>[2x]MNILKHFPSYVGPSKIRTLVIPIGHWTRKEFNNAVQKLSEFNEIHLSDVTPIDSPIFTPQGFPHGKLFFDFLTIDHDDALELFLYDFEPFRKTFVIIGLVNDYSDPLTNLNFMKEKYPTLISPNLVYASSTPTKELEQTIDTMENVFASSPDMQKNIETIMCDIARNFLTALNSYYSSYKHVTLRSPGAIGGNAVLKTTLIRQNSYTSSSSSTPMSAVQSSVSSSSKAGSVTTASKRLSSFEMTTNSLKRSASLKLATTLSTSENRSQQKSLGRQMKILGNFQLLAGRYVDALNSFVDAITTLYKVRDYLWLGSALDGISICFLLLSYLGLSYQIPQIVSLICPVEKLNFESSSTGISPVDSNSKATASTTASSTPRNSISIAAMQSPRNSIMSLSAPALNIDVENINLPLLIKCISDKVLYYYDLSLMHNSEYAPQVVYCEFLLKTLTFMTSCYKSSEFSKDVLDNIVKNQHRALSDIPNSPMFPRFEVYFYSNKLFELQLKEMQVEAQIKIYSTMAEVYRLLGYKRKQLFVLRLLMVALLATPNKIAWHPDYRTLIDTIIELLNINESEAKINVDDPSQSTWLILQKKILQLCIKVSRKINDFEYVAKFSSILITKYTHLLNQSEQDALFKEYIQPSITNESITSYWDPFILREVVINRILDSDPTSNEIPLESDVSSLESLENRQKTQDINPQEVFNPFKRVQPTSFVSNNSTKVPILVFLVGDKAEFTCRVQNPFKFDFTINDIQLDEEISEFCEIDRKAVSYSGPYNVKAESIRSITLPLIIKKPTYKKIYEISCLKISILKLPLQKFDIINDSRRSNPVEEEAEYSKCIYGKLKIKILPEQPQLELLSTSKMTRNSWMMLDGTKTDFHITVRNKSLSCAINHIKIIPMNNIEQMLKPDYWKKMPPDDLYIMEKQLDWLSKSCVRIIKLPTVIKPNETITFDLELDNTAVPFNFTGFDLLIEYGMSATDESCIYLKKLSIPYEVTLRRTIEVPSMDIIPLNELFSSQVENVDWIEYVMSKIRAESNLHSRDFILLLLDFRNSWIDGIKLNVQFEDFTSNEYHVEASHTSRIIVPIKKIDYKKYNFENTPIPRIYPGRQFIQSGLNEEQTIEMRQKFWCREHIISKLKCNWKLTTDQSVTGSVDFNKFIEKFDHKMVYTIYPGRLFYGVQLLLDEPKVKVGEIINLKIITEPTSTCRRKQNSTVNFLDIVIFDSKTSKILPRSNRRILYNGSLTKPISTTKVSEINLEIIPIEKGRYEFSVCISKSNNQDGIIQFDSENVILSVI;>MDKEIYCGSVPVSYFDPFDLFESLRPEFQQILPLDNIHWKAFDGTVRTVNRLPIELIPEGRGEADKSNDEQPFIRFLIVNCISIDQYRAKVRPLVRQWLPNLESVSSSTGEKMIYKPIILLYANSEVVDSNLFKSVSLMEKFGKDFPHVQTLEVRSVYRSPKERQEFWNQFSQKIKASVLSIFQKRLTHLQHSLANLQKGNNFEEQLLTREKLYELYVVFNILEDASLELQKIKKEILRRNMNMPDGKLQVPFESSSKSDESLGSIIIEGTLDKFQLHKYFFIRRLRLLKLEDQTLTAFVGAFQLIKNFIESISIEYRKSVRLLEFKHYFITSMLSYFEFENVSNPLLCEIKAELLMLKRDNWVQGVMATSGYRLMDKNYPNSDVKYKFDLLKETFVDETVFQENFLTLTKEILSLFNKCEGKRQRIVDILSIEIGLLYYQGKKYEEAVSLFLSCYEYYTQTNWNSIGLKILQVFIDSLSHCPKLDVLQIDGESVSASAVLTNAFLNILKLCKDNDSKEIWWKKFMDLQMKNNIHLMYPLDGLFEVTLNSKVHLARANVSAIEVNLKSYGFPEDISTKTMRLSLKNMGGDVIVFGASDFLLKKGENKLILECRDIMYGEFSLLSFEIIVEGITFVKEFPENQDEFIVVPEIYCKESTKVLVKQAHNLNLGEYALELKSVQSDALESLQVEVEVQKNIGNMKNLPVSFSMDEIQARKRYNTPFENVRLEYYLLDQITAFDLIIKTSFTKKNDQGTFGETKKVRIQCYLQLSVSVEDIFKKDIFFFKFLLNSSVREEPVILYSSELSAPDTRNDYNIRGDYIATTPALITFDGNESFINCYEITANNNFDSKDIFNLKVRYNTLKEQLDCFITDAVLIEGDVEWFILFEKWKTFWELEILKKLKYDYDAFKENRIIRLLKTS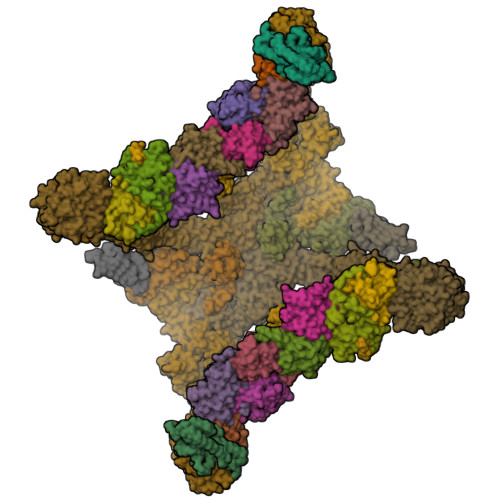IDLNKTKSKIRNLCIEKAVLDKILICLNKVSRGIAVCNTDMDEYVRNLVPKQLTVPVQLPGFEQFFHVQFEQMETSHDALHDTIATIGNSLSYTVIVENLSGQWGQDVIDDGGYIFEILSSNEWLIHGQKRCAIKEKRKEFEVHLIPLKKGYLNFPRVEITNINGKSCRVDHSNAFESILIFAA[2x];>[2x]MECFVPLRCDLDGSNIEQLRQSHLSRKFIIFDEQLNLWLWFQGNSQENKRFVLQNMIILINEAQVTRTSTIDDYFTQVENNENLWRLKNDCCSKILFKSNVVMNNGYNNQIKFVFEYKSVDANFNNQDSLQDPQAKYTLDKYSSEEILPSFEPVYSWSSAATKSSKNTNNHLEKNNRATHRVSSKNSEVHEADVSRNPNTFTLKLQYPIFSLLNMRLRNISLKSEHCILSSLDFQTSKASEQLTKKFIYPQEHNSFLKLNFQEISYKLIDGTSQIELDPICPLKVPLTAFSYDSISATFKLVLLPKSTQPHRVKITLAYELELHPNLKLPVRTSWETEVTLKRSMPISSTSSQYSSNNNNTNHSASFNGAANNVNSGGLANLRLGGVSSSRFSLGAASTTSLVNSKLSNVKFKFINSNIKVIKGEKFTMRLQIINSSSSPLDLVVYYNNTINPIPSANNVRNSNGINNCGMNNGTIPNSPLTLENQYQLHNKYRKIAEGIILLSNDYKIPVVPPRETYFADLRFIGIMSGYYGTLSGLKVLDLNTNELIEVGNGASVLIQ;>MSLRPCFVSLIDESDKPILIYVPNEAENEMNDVLKYNVLSNISLDYFESALVEWHSLDSKPLLKSIFQLEGVSVFAMLIKQTGLKIVIGFEQKSLSGADDEFEAINQIFETVRKIYIRVKCNPLLVSGDEKSIIKSLERKFDELFISTEVEL[2x];>[2x]MSSTHSNNVGHPQSSPQGPLTEQQRAQQQYQIFENSLPKVSQSVYQMLLNEMVPLAMGIERQISGDVISSDSNVTSENGNINNMIKRLKIEEHHTVDIIRSHNLIHELYKADEEEKEKVLARLRNIGFQIGLKLSELLIFSNNPNLKFKEMDLLLIMKFICRDVWKQIFGKQIDNLKTNHRGTFYLLDYDYRPIQSFSLEEDAKNEELKMIEPFLEIPVGIIRGVLSSLGYSSEEVICLASFIDRPTDRPKTAFPKGVSFHVQVTMPQ;>MVSTTQSRSLKAMGEEIWKNKTEKINTELFTLTYGSIVAQLCQDYERDFNKVNDHLYSMGYNIGCRLIEDFLARTALPRCENLVKTSEVLSKCAFKIFLNITPNITNWSHNKDTFSLILDENPLADFVELPMDAMKSLWYSNILCGVLKGSLEMVQLDCDVWFVSDILRGDSQTEIKVKLNRILKDEIPIGED[4x];>[2x]MGIYSFWIFDRHCNCIFDREWTLASNSASGTINSKQNEEDAKLLYGMIFSLRSITQKLSKGSVKNDIRSISTGKYRVHTYCTASGLWFVLLSDFKQQSYTQVLQYIYSHIYVKYVSNNLLSPYDFAENENEMRGQGTRKITNRNFISVLESFLAPMVNQ;>[2x]MAIETILVINKSGGLIYQRNFTNDEQKLNSNEYLILASTLHGVFAIASQLTPKALQLTQQTNIENTIPYIPYVGMSSNRSDTRNGGGNNNKHTNNEKLGSFKGDDFFKEPFTNWNKSGLRQLCTDQFTMFIYQTLTGLKFVAISSSVMPQRQPTIATTDKPDRPKSTSNLAIQIADNFLRKVYCLYSDYVMKDPSYSMEMPIRSNLFDEKVKKMVENLQ;>[2x]MSQRIIQPSASDQQFPGKSDGYEYTVGPKQAITSEASTTYIPSRIYSESLLFKRQEASLSAMAFLFQEMISQLHRTCKTAGDFETKLSDYGHNIGIRLLELLNFRASVSPSSLPRASAFLSQNESSSKLSNASNSPGMLANSSTATSASANERLQEKQTESLSNYITKMRRRDLKILDILQFIHGTLWSYLFNHVSDDLVKSSERDNEYMIVDNFPTLTQFIPGENVSCEYFVCGIIKGFLFNAGFPCGVTAHRMPQGGHSQRTVYLIQFDRQVLDREGLRFG;>MPQYFAIIGKKDNPVYEIEFTNAENPQGFPQDLKELNPFILHASLDIVEDLQWQINPTSQLNGNGGNGSNGGGGFLRSRAVNNTDNCYLGKVDHFYGLAITAYISYSGMKFVMIHGNSANSSVVIDDNNMRSFYQEVHELYVKTLMNPFYKITDPIRSPAFDSRVRTLARKHLSK[2x];>[2x]MSNEDYGYDYDYLFKIVLIGDSGVGKSNLLSRFTTDEFNIESKSTIGVEFATRTIEVENKKIKAQIWDTAGQERYRAITSAYYRGAVGALIVYDISKSSSYENCNHWLTELRENADDNVAVGLIGNKSDLAHLRAVPTDEAKNFAMENQMLFTETSALNSDNVDKAFRELIVAIFQMVSKHQVDLSGSGTNNMGSNGAPKGPTISLTPAPKEDKKKKSSNHHHHHHH>GSPGENLKHIITLGQVIHKRCEEMKYCKKQCRRLGHRVLGLIKPLEMLQDQGKRSVPSEKLTTAMNRFKA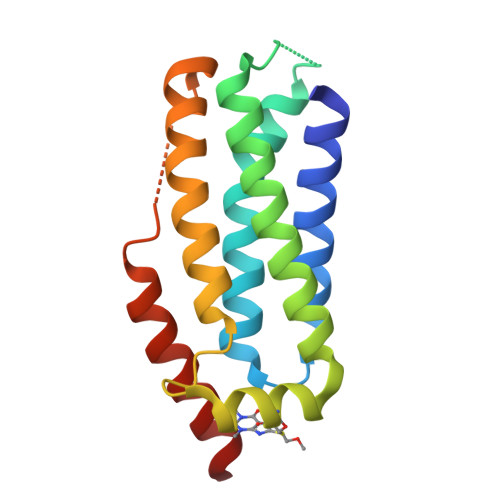ALEEANGEIEKFSNRSNICRFLTASQDKILFKDVNRKLSDVWKELSLLLQVEQRMPVSPISQGASWAQEDQQDADEDRRAFQM[2x]> ASAAEAAAEQARPYAIPAGQLGDVLNRFAREAGITLSATPAQTGGYSSQGLRGSFTVQQGLARLLADTPLEAEDQGDGSFVLREAPAKDGDVLNMQAVEVFALGNNLGSTDGYLATHSQIATKTSKPLLETSQTVSVITREQIDDTASKTVQQAMRYTPGIFTGQVGASNRYDYVVMRGFADNSVDNIYLDGLKAMGDSGTFSSMQVDPYFLERIDVLKGPSSVLYGRSLPGGLVALTSKKPLYEDYRQITGSIGNMGQKEMGFDFSGPLDEEKRIAYRLIGLGKGSDTQFDHVKEERYAIAPTLAIDFSDDTTLTLQGYLQHDPNGGYHGGVPADGTLSHHNGRHISREFFDGEPSKDDFDRTQRMFGYQLEHRIDDVWSARQNFRYLDSDVDLSQVYAYGWSASEPNKLNRYFSGAREHLQAYIVDNMLQAEFATGAARHT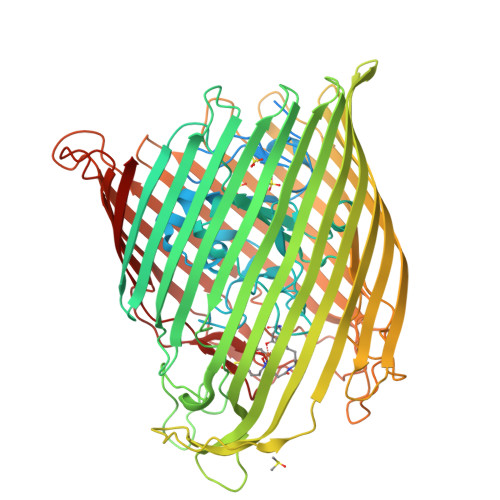LLTGLDYQRRRTVVDWRSGSASALDAFNPVYGDDAISYFPDDNHTRRLEQTGVYLQDLIDIDQWRFSLGLRQDWVSVTDKNRSTGSKADDDWEKFTGRIGALYLFDNGLAPYVSYSESFNPNAYSDASGTPLAPTEGKQWELGLKFQAPGSNSFYTASLFHITQENVASKEPQDNFYTSVGEVRSQGLELEAHTQLSDNLKLLGSYTYTDITYTKSLDGNQGHTPNQAPKHMASLWADYAFDAGPLSGLSIGGGARYVGETWADKENTLRVPDYTLVDARIGYDLGKLGLKGLDVSLNANNLLDKDYVASCYSLDFCYFGEKRNVTATVNYQF> MKEFYLTVEQIGDSIFERYIDSNGRERTREVEYKPSLFAHCPESQATKYFDIYGKPCTRKLFANMRDASQWIKRMEDIGLEALGMDDFKLAYLSDTYNYEIKYDHTKIRVANFDIEVTSPDGFPEPSQAKHPIDAITHYDSIDDRFYVFDLLNSPYGNVEEWSIEIAAKLQEQGGDEVPSEIIDKIIYMPFDNEKELLMEYLNFWQQKTPVILTGWNVESFAIPYVYNRIKNIFGESTAKRLSPHRKTRVKVIENMYGSREIITLFGISVLDYIDLYKKFSFTNQPSYSLDYISEFELNVGKLKYDGPISKLRESNHQRYISYNIIAVYRVLQIDAKRQFINLSLDMGYYAKIQIQSVFSPIKTWDAIIFNSLKEQNKVIPQGRSHPVQPYPGAFVKEPIPNRYKYVMSFDLTSFYPSIIRQVNISPETIAGTFKVAPLHDYINAVAERPSDVYSCSPNGMMYYKDRDGVVPTEITKVFNQRKEHKGYMLAAQRNGEIIKEALHNPNLSVDEPLDVDYRFDFSDEIKEKIKKLSAKSLNEMLFRAQRTEVAGMTAQINRKLLINSLYGALGNVWFRYYDLRNATAITTFGQMALQWIERKVNEYLNEVCGTEGEAFVLYGDTDSIYVSADKIIDKVGESKFRDTNHWVDFLDKFARERMEPAIDRGFREMCEYMNNKQHLMFMDREAIAGPPLGSKGIGGFWTGKKRYALNVWDMEGTRYAEPKLKIMGLETQKSSTPKAVQKALKECIRRMLQEGEESLQEYFKEFEKEFRQLN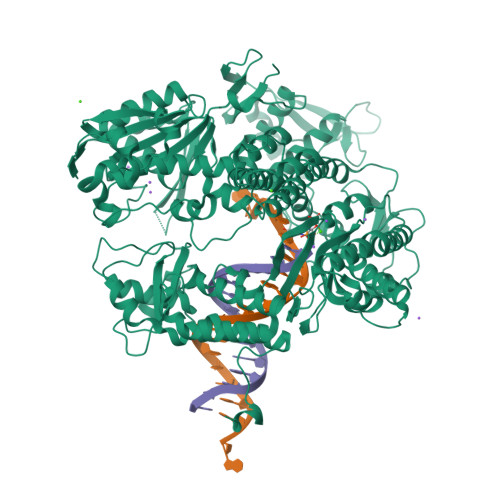YISIASVSSANNIAKYDVGGFPGPKCPFHIRGILTYNRAIKGNIDAPQVVEGEKVYVLPLREGNPFGDKCIAWPSGTEITDLIKDDVLHWMDYTVLLEKTFIKPLEGFTSAAKLDYEKKASLFDMFDF The long-wavelength beamline I23 at Diamond Light Source overcomes these limitations and extends the accessible wavelength range to λ = 5.9 Å. In this study, we report the determination of diverse protein structures by experimental phasing techniques carried out at long wavelengths on beamline I23 at Diamond Light Source using S, Ca, K, Cl, V, I, Cd, and P as anomalous scatterers. Native-SAD uses light atoms naturally occurring in proteins or bound to proteins. We demonstrate that long-wavelength native-SAD has become a very compelling technique, where a low multiplicity dataset from a single crystal can be sufficient for successful structure determination, making it a general vehicle of choice for experimental phasing.

Using this protocol, we selected 10 projects solved by S-SAD phasing at the beamline, including soluble and membrane proteins. Structures varied in size with molecular weights ranging from 14 to 114 kDa, sulfur contents varied between 0.9 and 6.5%, and diffraction resolution from 1.8 (detector limited) to 3.4 Å. The overall multiplicity for these datasets was below 26, which is four times lower than the multiplicity typically needed for S-SAD at shorter wavelengths (100)10.

>[2x]LDLFTLSFSPDLSIASEAEQLTLQSKDDRLILEHPQPGLRTALEQLKQGNLTLAQLTELVSEQDGVEAGITFASELEKLVDLGWICHSVLPLITAIPIAKDYELNVPDSSWQTTAIALSRFAFLHQDLQQLVLESPRSKSKLVILDWRVGAVIAKLAQSDRGFIFATSADSLLADLSLELEELKRLFALLIATQMMDLEPEDETITQWKFHNLLFHHYTRLGRLDNSRKLNLPVFEHRDRYPYVKPVISTQAIPLVKPDLTALATTDMTLTEAIETRRSIREYSDQPITLAQLGEFLYRCARVKAVYTLPEDPMQVGESTTRPYPSGGALYELEIYPLVHQCGDLAAGLYHYQPLSHTLHPVADWTPEVESLVYDAWRATGQQSIPQIVLIITARFGRLFWKYHDIAYSLILKHVGVLYQTFYLVATAMQLAPSAIGAGNTTKFCQIAGLNPDEEASVGEFSLGAAKPQQQS> MSADAQSFLNRVCGVSAARLTPCGTGTSTDVVYRAFDIYNDKVAGFAKFLKTNCCRFQEKDEDDNLIDSYFVVKRHTFSNYQHEETIYNLLKDCPAVAKHDFFKFRIDGDMVPHISRQRLTKYTMADLVYALRHFDEGNCDTLKEILVTYNCCDDDYFNKKDWYDFVENPDILRVYANLGERVRQALLKTVQF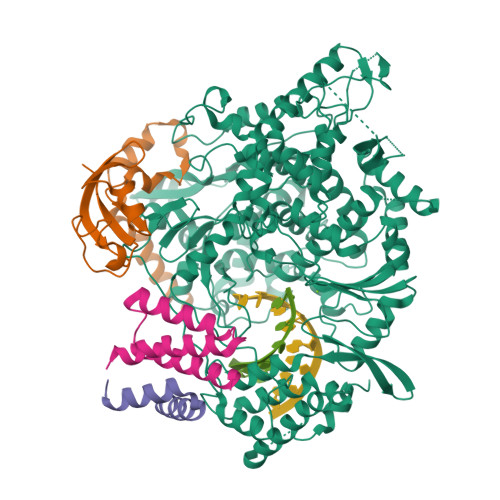CDAMRNAGIVGVLTLDNQDLNGNWYDFGDFIQTTPGSGVPVVDSYYSLLMPILTLTRALTAESHVDTDLTKPYIKWDLLKYDFTEERLKLFDRYFKYWDQTYHPNCVNCLDDRCILHCANFNVLFSTVFPPTSFGPLVRKIFVDGVPFVVSTGYHFRELGVVHNQDVNLHSSRLSFKELLVYAADPAMHAASGNLLLDKRTTCFSVAALTNNVAFQTVKPGNFNKDFYDFAVSKGFFKEGSSVELKHFFFAQDGNAAISDYDYYRYNLPTMCDIRQLLFVVEVVDKYFDCYDGGCINANQVIVNNLDKSAGFPFNKWGKARLYYDSMSYEDQDALFAYTKRNVIPTITQMNLKYAISAKNRARTVAGVSICSTMTNRQFHQKLLKSIAATRGATVVIGTSKFYGGWHNMLKTVYSDVENPHLMGWDYPKCDRAMPNMLRIMASLVLARKHTTCCSLSHRFYRLANECAQVLSEMVMCGGSLYVKPGGTSSGDATTAYANSVFNICQAVTANVNALLSTDGNKIADKYVRNLQHRLYECLYRNRDVDTDFVNEFYAYLRKHFSMMILSDDAVVCFNSTYASQGLVASIKNFKSVLYYQNNVFMSEAKCWTETDLTKGPHEFCSQHTMLVKQGDDYVYLPYPDPSRILGAGCFVDDIVKTDGTLMIERFVSLAIDAYPLTKHPNQEYADVFHLYLQYIRKLHDELTGHMLDMYSVMLTNDNTSRYWEPEFYEAMYTPHTVLQLEHHHHHH;>MAIASEFSSLPSYAAFATAQEAYEQAVANGDSEVVLKKLKKSLNVAKSEFDRDAAMQRKLEKMADQAMTQMYKQARSEDKRAKVTSAMQTMLFTMLRKLDNDALNNIINNARDGCVPLNIIPLTTAAKLMVVIPDYNTYKNTCDGTTFTYASALWEIQQVVDADSKIVQLSEISMDNSPNLAWPLIVTALRANSAVKLQLEHHHHHH[2x];> MSKMSDVKCTSVVLLSVLQQLRVESSSKLWAQCVQLHNDILLAKDTTEAFEKMVSLLSVLLSMQGAVDINKLCEEMLDNRATLQLEHHHHHH>[2x]MHVSSLKVVLFGVCCLSLAACQTPAPVKNTASRSAASVPA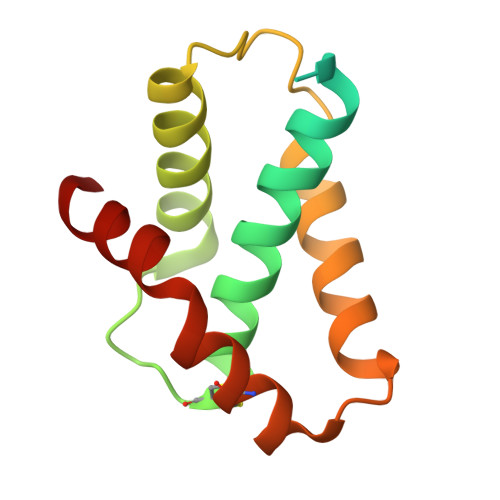NEQISQLASLVAASKYLRVQCERSDLPDDGTILKTAVNVAVQKGWDTGRYQSLPQLSENLYQGLLKDGTPKATQCSSFNRTMTPFLDAMRTVR> MKHHHHHHSAGLEVLFQGPGTGSEFELMMFGKKKNNGGSSTARYSAGNKYNTLSNNYALSAQQLLNASKIDDIDSMMGFERYVPPQYNGRFDAKDIDQIPGRVGWLTNMHATLVSQETLSSGSNGGGNSNDGERVTTNQGISGVDFYFLDEEGGSFKSTVVYDPYFFIACNDESRVNDVEELVKKYLESCLKSLQIIRKEDLTMDNHLLGLQKTLIKLSFVNSNQLFEARKLLRPILQDNANNNVQRNIYNVAANGSEKVDAKHLIEDIREYDVPYHVRVSIDKDIRVGKWYKVTQQGFIEDTRKIAFADPVVMAFAIATTKPPLKFPDSAVDQIMMISYMIDGEGFLITNREIISEDIEDFEYTPKPEYPGFFTIFNENDEVALLQRFFEHIRDVRPTVISTFNGDFFDWPFIHNRSKIHGLDMFDEIGFAPDAEGEYKSSYCSHMDCFRWVKRDSYLPQGSQGLKAVTQSKLGYNPIELDPELMTPYAFEKPQHLSEYSVSDAVATYYLYMKYVHPFIFSLCTIIPLNPDETLRKGTGTLCEMLLMVQAYQHNILLPNKHTDPIERFYDGHLLESETYVGGHVESLEAGVFRSDLKNEFKIDPSAIDELLQELPEALKFSVEVENKSSVDKVTNFEEIKNQITQKLLELKENNIRNELPLIYHVDVASMYPNIMTTNRLQPDSIKAERDCASCDFNRPGKTCARKLKWAWRGEFFPSKMDEYNMIKRALQNETFPNKNKFSKKKVLTFDELSYADQVIHIKKRLTEYSRKVYHRVKVSEIVEREAIVCQRENPFYVDTVKSFRDRRYEF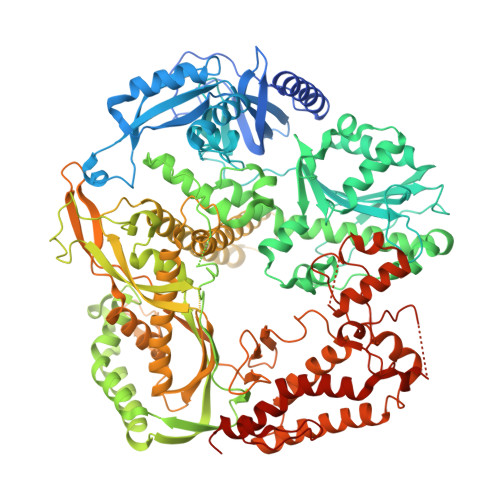KGLAKTWKGNLSKIDPSDKHARDEAKKMIVLYDSLQLAHKVILNSFYGYVMRKGSRWYSMEMAGITCLTGATIIQMARALVERVGRPLELDTDGIWCILPKSFPETYFFTLENGKKLYLSYPCSMLNYRVHQKFTNHQYQELKDPLNYIYETHSENTIFFEVDGPYKAMILPSSKEEGKGIKKRYAVFNEDGSLAELKGFELKRRGELQLIKNFQSDIFKVFLEGDTLEGCYSAVASVCNRWLDVLDSHGLMLEDEDLVSLICENRSMSKTLKEYEGQKSTSITTARRLGDFLGEDMVKDKGLQCKYIISSKPFNAPVTERAIPVAIFSADIPIKRSFLRRWTLDPSLEDLDIRTIIDWGYYRERLGSAIQKIITIPAALQGVSNPVPRVEHPDWLKRKIAT>MTMQIKIKYLDETQTRISKIEQGDWIDLRAAEDVTIKKDEFKLVPLGVAMELPEGYEAHVVPRSSTYKNFGVIQTNSMGVIDESYKGD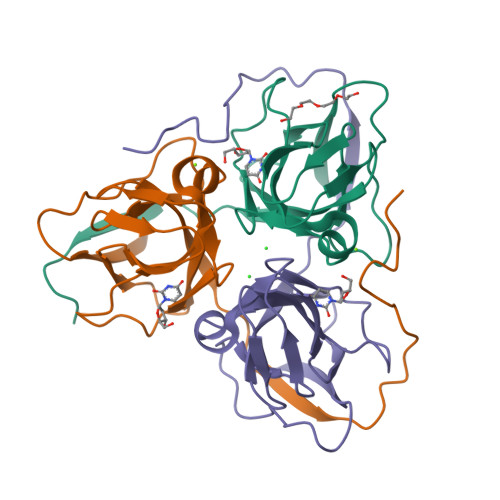NDFWFFPAYALRDTEIKKGDRICQFRIMKKMPAVELVEVEHLGNEDRGGLGSTGTK[3x]> MNHKVHHHHHHHHMATFISVQLKKTSEVDLAKPLVKFIQQTYPSGGEEQAQYCRAAEELSKLRRAAVGRPLDKHEGALETLLRYYDQICSIEPKFPFSENQICLTFTWKDAFDKGSLFGGSVKLALASLGYEKSCVLFNCAALASQIAAEQNLDNDEGLKIAAKHYQF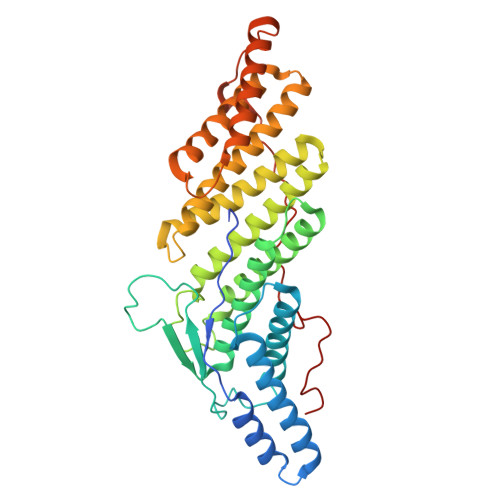ASGAFLHIKETVLSALSREPTVDISPDTVGTLSLIMLAQAQEVFFLKATRDKMKDAIIAKLANQAADYFGDAFKQCQYKDTLPKEVFPVLAAKHCIMQANAEYHQSILAKQQKKFGEEIARLQHAAELIKTVASRYDEYVNVKDFSDKINRALAAAKKDNDFIYHDRVPDLKDLDPIGKATLVKSTPVNVPISQKFTDLFEKMV>[2x]MSLVVFPFKHEHPEVLLHNVRVAA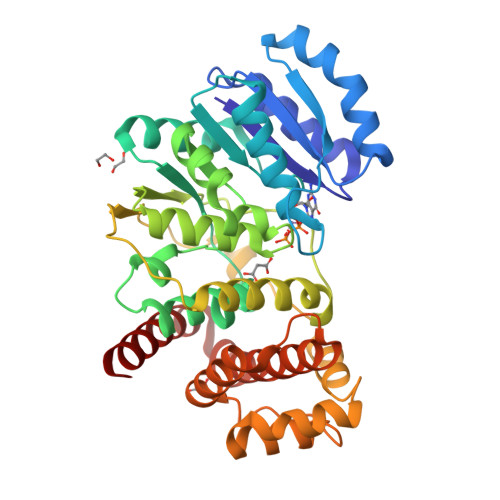AHPRVHEVLCIGYERDQTYEAVERAAPEISRATGTPVSVRLQERLGTLRPGKGDGMNTALRYFLEETQWERIHFYDADITSFGPDWITKAEEAADFGYGLVRHYFPRASTDAMITWMITRTGFALLWPHTELSWIEQPLGGELLMRREVAAMLYEDERVRRRSDWGIDTLYTFVTVAAGVSIYECYIPEGKAHRLYGGLDDLRTMLVECFAAIQSLQHEVVGQPAIHRQEHPHRVPVHIAERVGYDVEATLHRLMQHWTPRQVELLELFTTPVREGLRTCQRRPAFNFMDEMAWAATYHVLLEHFQPGDPDWEELLFKLWTTRVLNYTMTVALRGYDYAQQYLYRMLGRYRYQAALEN> MICRFIDTHCHFDFPPFSGDEEASLQRAAQAGVGKIIVPATEAENFARVLALAENYQPLYAALGLHPGMLEKHSDVSLEQLQQALERRPAKVVAVGEIGLDLFGDDPQFERQQWLLDEQLKLAKRYDLPVILHSRRTHDKLAMHLKRHDLPRTGVVHGFSGSLQQAERFVQLGYKIGVGGTITYPRASKTRDVIAKLPLASLLLETDAPDMPLNGFQG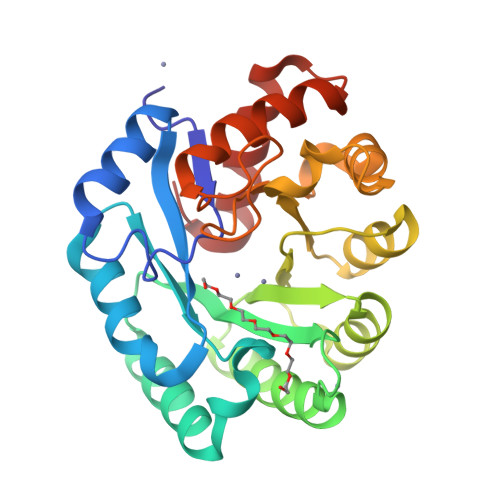QPNRPEQAARVFAVLCELRREPADEIAQALLNNTYTLFNVP>[3x]MASSRRESINPWILTGFADAEGSFGLSILNRNRGTARYHTRLSFAIVLHNKDKSILENIQSTWKVGIITNDGDRYVRLRVTRFEDLKVIIDHFEKYPLVTQKLGDYKLFKQAFSVMENKEHLKENGIKELVRIKAKMNWGLNDELKKAFPENISKERPLINKNIPNFKWLAGFTSGDGSFFVRLRKSNVNARVRVQLVFEISQHIRDKNLMNSLITYLGCGHIYEGNKSERSWLQFRVEKFSDIN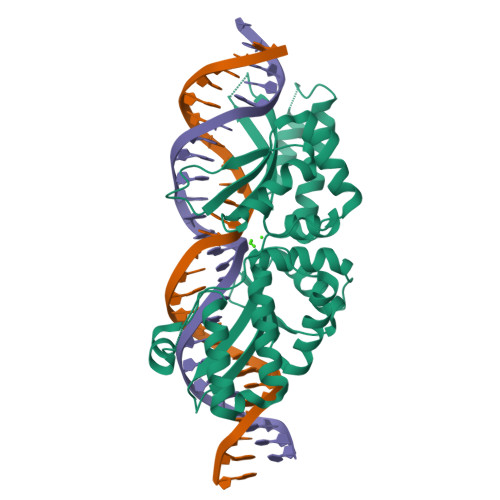DKIIPVFQENTLIGVKLEDFEDWCKVAKLIEEKKHLTESGLDEIKKIKLNMNKGR butyl alpha-D-mannopyranoside 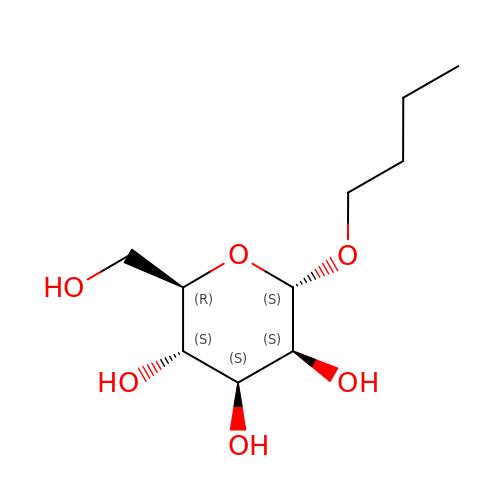| C10 H20 O6 | BZANQLIRVMZFOS-ZJDVBMNYSA-N>GPGSEFSRHSEKIAI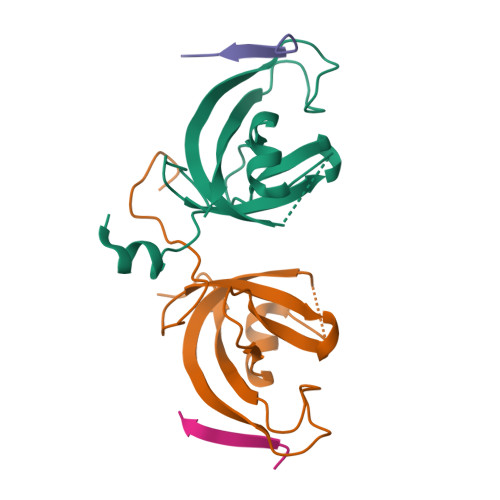RDFQVGDLVLIILDERHDNYVLFTVSPTLYFLHSESLPALDLKPGEGASGASRRPWVLGKVMEKEYCQAKKAQNRFKVPLGTKFYRVKAVSWNKKV[2x];>[2x]GPGSEQDDDIEVIVDET>GSNFCDSKCKLRCSKAGLADRCLKFCGICCEECKCVPSGTYGNKHECPCYRDKKNSKGKSKCP[2x];>GSNFCDSKCKLRCSKAGLADRCLKYCGICCEECKCVPSGTYGNKHECPCYRDKKNSKGKSKCP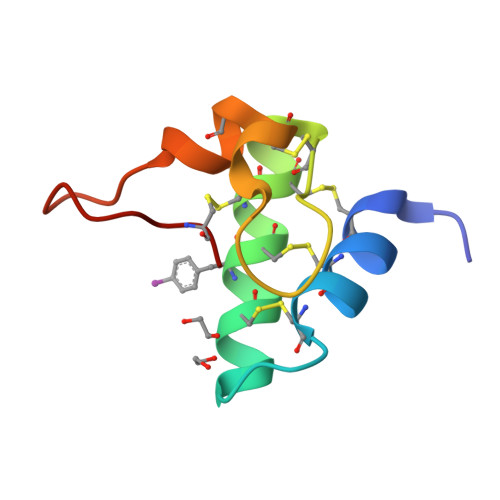[2x]> GSHMAEKPHMNLVVIGHVDHGKSTLVGHLLYRLGYIEEKKLKELEEQAKSRGKESFKFAWILDKMKEERERGITIDLTFMKFETKKYVFTIIDAPGHRDFVKNMITGASQADAAILVVSARKGEFEAGMSTEGQTREHLLLARTMGIEQIIVAVNKMDAPDVNYDQKRYEFVVSVLKKFMKGLGYQVDKIPFIPVSAWKGDNLIE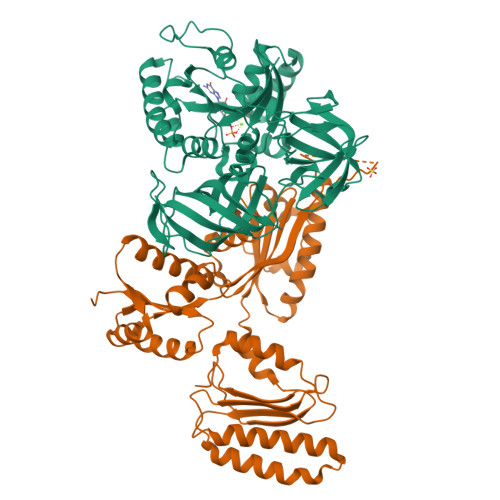RSPNMPWYNGPTLVEALDQLQPPAKPVDKPLRIPVQNVYSIPGAGTVPVGRVETGVLRVGDKVVFMPPGVVGEVRSIEMHYQQLQQAEPGDNIGFAVRGVSKSDIKRGDVAGHLDKPPTVAEEFEARIFVIWHPSAITVGYTPVIHVHTASVSSRIIEIKAKLDPKTGQVVEQNPQFLKAGDAAIVRFKPVKPLVVEKFSEIPQLGRFAMRDMNRTVGIGIVTDVKPAKVDIKAK;> MSQGRLEERLTISKRELARLLKELKKWSAPATVLLSLYIPPGRPLSDVMTLLRQEYSITDNIKLKRTRQAVKRALSAAMDRLQMLTSTPPNGLVLFCGEDMSTGKFECFMFSPPEPIRVFYYRTDKRFITDFLEDMVEDNNAIGIIIVERDQATIGLLKGARLEVLKELEGFVPGKHKMGGQSQRRYERIIEQMVDEFFKKVGEEASNLLVPLAEKGVLKGVIVAGPGLAKQEFVEGNYLDYRLKKILAPELVDVAYQGLQGLKEAVMKAEKVVEAQMYRDAVNAMEEFKLHLAKGTGMIVYGEKDVEAALEMGAVKTLLIHESREDLEEWVEKAKSSGAQVIVVPESLAEAEWFLKTFGGLAGILRFRISTV>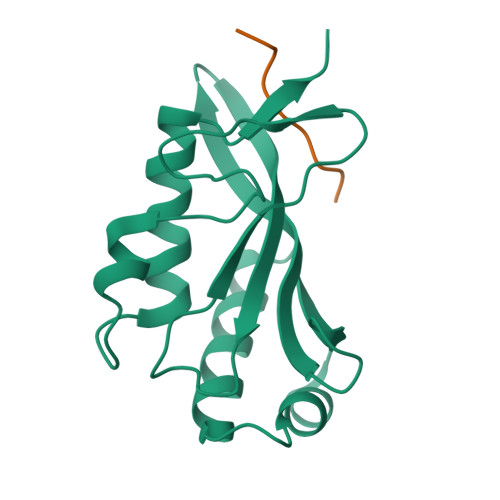 GAMGSAVSESQLKKMVSKYKYRDLTVRETVNVITLYKDLKPVLDSYGTGSRELMNLTGTIPVPYRGNTYNIPICLWLLDTYPYNPPICFVKPTSSMTIKTGKHVDANGKIYLPYLHEWKHPQSDLLGLIQVMIVVFGDEPPVFSRP;> PEATAPPEE2,3-di(butanoyloxy)propyl 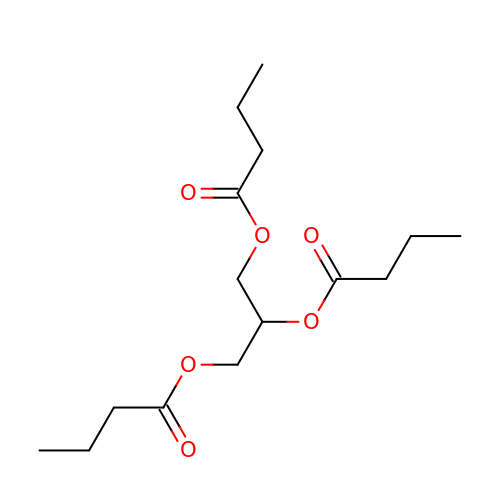butanoate | C15 H26 O6 | UYXTWWCETRIEDR-UHFFFAOYSA-N> SMAEDTGVRVELAEEDHGRKSTIALRLWVEDPKKLKGKPKDNGAIEFTFDLEKETPDEVAQEMIESGF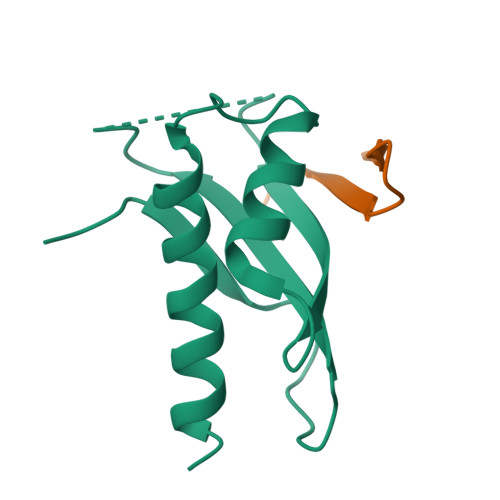FHESDVKIVAKSIRDRVALIQWRRERIWPA;> LTQVVHSAGRRFIVSPVPESRLR2-{(3R,4S)-3-[(5-{[benzyl(methyl)amino]methyl}-1,2-oxazol-3-yl)methyl]piperidin-4-yl}-N-(1,3-thiazol-2-yl)acetamide | C23 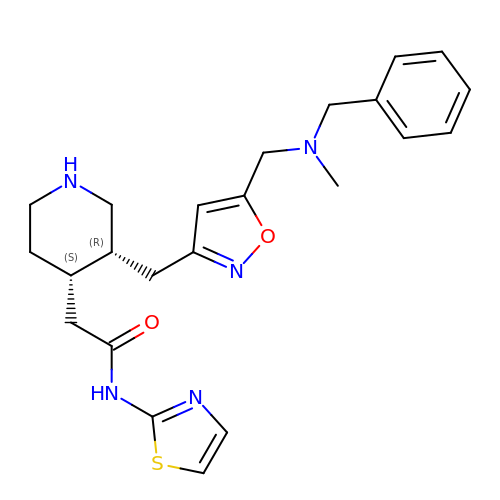H29 N5 O2 S | UCRRMFAAQQXDGH-OALUTQOASA-N>[24x]ATKKAVAVLKGNSNVEGVVTLSQDDDGPTTVNVRITGLAPGLHGFHLHEYGDTTNGCM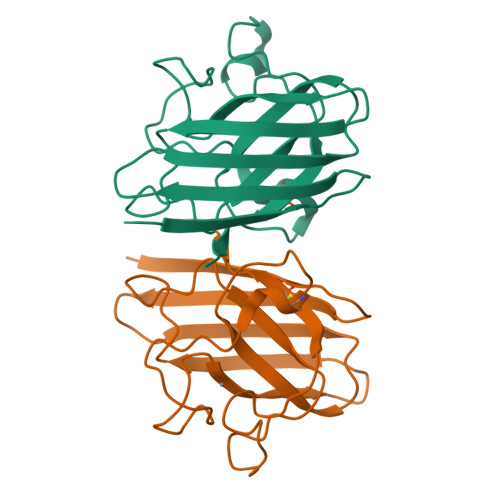STGAHFNPNKLTHGAPGDEIRHAGDLGNIVANADGVAEVTLVDNQIPLTGPNSVVGRALVVHELEDDLGKGGHELSLTTGNAGGRLACGVVGLTPI> MVVKKRKLATEAGGSDERPKYLPGKHPKNQEKTPHVDYNAPLNPKSELFLDDWHIPKFNRFISFTLDVLIDKYKDIFKDFIKLPSRKFHPQYYYKIQQPMSINEIKSRDYEYEDGPSNFLLDVELLTKNCQAYNEYDSLIVKNSMQVVMLIEFEVLKAKNLKRNYLINSEV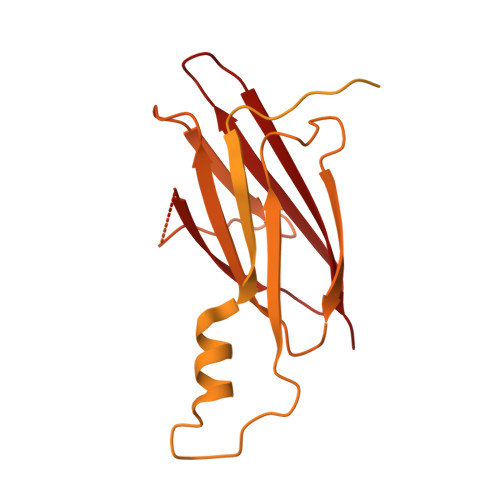KAKLLHYLNKLVDATEKKINQALLGASSPKNLDDKVKLSEPFMELVDKDELPEYYEIVHSPMALSIVKQNLEIGQYSKIYDFIIDMLLVFQNAHIFNDPSALIYKDATTLTNYFNYLIQKEFFPELQDLNERGEINLEFDKFEFENYLAIGGGGPAAAGALAISALDNDIEPESNREDLIDQADYDFNHFEGLGNGYNRSLLTEDYLLNPNNFKKLIAKPETVQSEVKNERSTTSDIEKTNSLESEHLKIPKYNVIKSMQKEMQSLSEQHTMEYKPYKLIQQIYIFSSKNLYSQATKPLLGSRPSCNQNWVEYIFNGNELSQNENAFSFMLQPMQTFLTLQSHLTSSLKDTETLLTINKEPVKSRTSNVNSNLSQPQQQENDVIGNDTKQDIENLTIGGGNNNDIVGNDNDKRNNITEIFDIRLSEGLNHLMFRCEDKISHETEFMNFWINVLP>[2x]MTKPLDGINVLDFTHVQAGPACTQMMGFLGANVIKIERRGSGDMTRGWLQDKPNVDSLYFTMFNCNKRSIELDMKTPEGKELLEQMIKKADVMVENFGPGALDRMGFTWEYIQELNPRVILASVKGYAEGHANEHLKVYENVAQCSGGAAATTGFWDGPPTVSGAALGDSNSGMHLMIGILAALEMRHKTGRGQKVA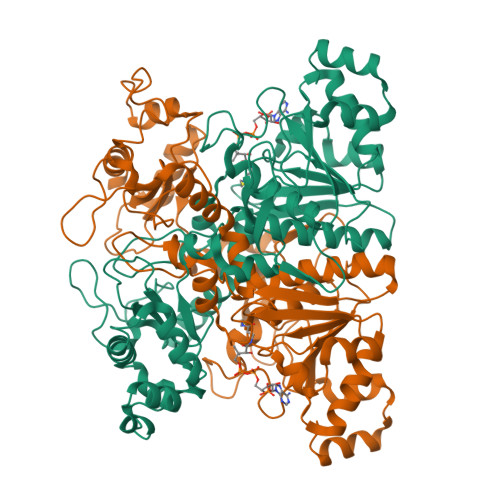VAMQDAVLNLVRIKLRDQQRLERTGILAEYPQAQPNFAFDRDGNPLSFDNITSVPRGGNAGGGGQPGWMLKCKGWETDADSYVYFTIAANMWPQICDMIDKPEWKDDPAYNTFEGRVDKLMDIFSFIETKFADKDKFEVTEWAAQYGIPCGPVMSMKELAHDPSLQKVGTVVEVVDEIRGNHLTVGAPFKFSGFQPEITRAPLLGEHTDEVLKELGLDDAKIKELHAKQVV>MSLRILIVDDEKLTRDGLIANINWKALSFDQIDQADDGINAIQIALKHPPNVLLTDVRMPRMDGIELVDNILKLYPDCSVIFMSGYSDKEYLKAAIKFRAIRYVEKPIDPSEIMDALKQSIQTVLQHQAQQDSEGHHHHHH[2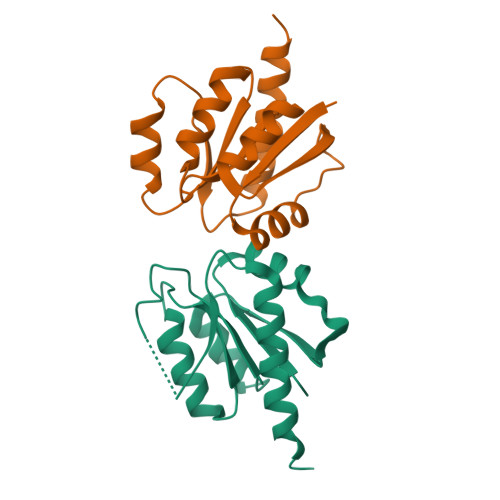x]> MHRVMGIETEYGISVPHQPNANAMAASSQVVNAYAPIGAPAQRQARWDFEEENPLRDARGFEVAREAADPSQLTDEDLGLANVILTNGARLYVDHAHPEYSTPEVTNPRDAVLWDKAGERIMAEAARRAADLPMGWTIQLYKNNTDNKGASYGCHENYLMNRSTPFADIVRHLIPFFVTRQVFCGAGRVGIGADGRGEGFQLSQRADFFEVEVGLETTLKRPIINTRDEPHADPEKYRRLHVIIGDANMSEIATYLKLGTTALVLAMIEDGFLSQDFSVESPVGALRAVSHDPTLRYQLRLHDGRRLTAVQLQMEYLEQARKYVEDRFGTDVDDMTRDVLDRWETTLVRLADDPMQLSRDLDWVAKLSILEGYRQRENLPWSAHKLQLVDLQYHDVRPDRGLYNRLVARGRMNLLVDEAAVRTAMHEPPNDTRAYFRGRCLAKFGAEIAAASWDSVIFDLPGRDSLQRVPTLEPLRGTRAHVGDLLDRCRSATELVAALTGGENLYFQ;> DAILDEIDDVLEENAEEFVRSYIQKGGQ

Pupylation is the post-translational modification of lysine side chains with prokaryotic ubiquitin-like protein (Pup) that targets proteins for proteasomal degradation in mycobacteria and other members of Actinobacteria. A single Pup ligase enzyme, PafA (proteasome accessory factor A), is responsible for modifying all pupylation substrate proteins and likewise a single depupylase enzyme, Dop (deamidase of Pup), removes Pup from Pup-protein adducts. Depupylase Dop is structurally homologous to Pup ligase PafA, although the two evolutionarily related enzymes catalyze opposing reactions. Rather, before the catalytic cycle of Dop can begin, Dop-mediated cleavage of ATP in the active site must take place to generate the Pi species important for catalysis.

Furthermore, in order to prevent the turnover of PupQ to PupE, the non-hydrolyzable ATP analog AMP-PCP was used, since ATPγS and AMP-PNP can still be hydrolyzed by Dop, albeit much more slowly. We obtained crystals of the enzyme in complex with the PupQ fragment and AMP-PCP and determined the structure at 1.65 Å resolution by molecular replacement. Upon binding to Dop, Pup undergoes a disorder-to-order transition adopting two well-resolved helices (helix 1: D44–V53; helix 2: N57–S64). However, Pup in complex with Dop exhibits a significantly more extensive network of interactions than Pup bound to the ligase PafA, with differences especially pronounced at the C-terminal residue of Pup. The C-terminal glutamine residue of Pup in the Dop-Pup complex is well defined in the electron density map and forms extensive interactions with Dop, whereas in the PafA-Pup complex, the C-terminus of Pup is poorly ordered, as indicated by the weak electron density, and only weakly forms a salt bridge with the side chain of R201. The Dop-Pup complex structure solved here shows that the loop preceding strand β7, referred to in the literature as α-loop (F208–K220), is involved in the binding of the C-terminal residue of Pup (Q71) through a strong hydrogen bond formed with T217. In the active site of the Dop-PupQ complex, the non-hydrolyzable ATP analog AMP-PCP displays strong and unambiguous density with an occupancy of about 72 %. Correspondingly, two of the three canonical Mg2+-binding sites (n1–n3) defined for the carboxylate-amine/ammonia ligase superfamily also show only partial occupancies (n2 and n3). The γ-phosphate of AMP-PCP is kinked slightly out of the active site and away from the side chain of the C-terminal Pup residue, likely due to the inability of the AMP-PCP-analogue-specific carbon atom between the β- and γ-phosphates to fill the empty coordination position of Mg2+ at the n3 site.>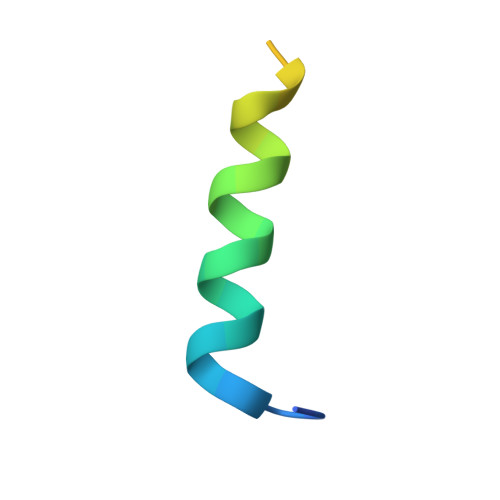 MATDSWAQAVDEQEAAAESISTLQISEKEEKP1-[[(1E)-2-(4-CHLOROPHENYL)ETHENYL]SULFONYL]-4-[[1-(4-PYRIDINYL)-4-PIPERIDINYL]METHYL]PIPERAZINE | C23 H29 Cl N4 O2 S | 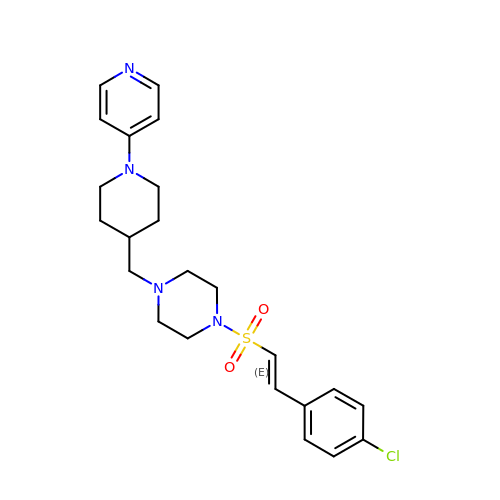ZOSSOFIFNGGDKG-GIJQJNRQSA-N>[2x]SMMELRVGNRYRLGRKIGSGSFGDIYLGTDIAAGEEVAIKLECVKTKHPQLHIESKIYKMMQGGVGIPTIRWCGAEGDYNVMVMELLGPSLEDLFNFCSRKFSLKTVLLLADQMISRIEYIHSKNFIHRDVKPDNFLMGLGKKGNLVYIIDFGLAKKYRDARTHQ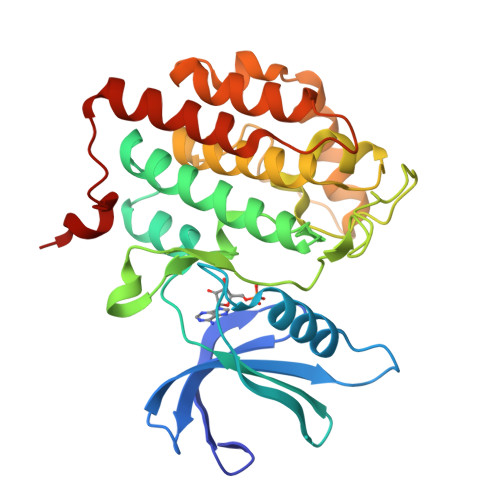HIPYRENKNLTGTARYASINTHLGIEQSRRDDLESLGYVLMYFNLGSLPWQGLKAATKRQKYERISEKKMSTPIEVLCKGYPSEFATYLNFCRSLRFDDKPDYSYLRQLFRNLFHRQGFSYDYVFDWNMLK>GSAAIIPPWLNIPENSRFFVIKSSSLKHVKRSF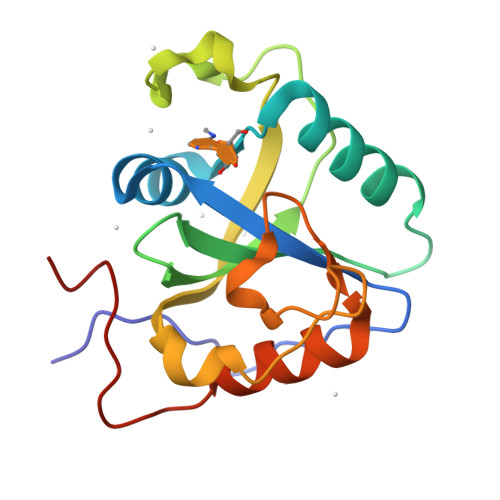YNGIWSSTHFGNKRLSEAYKKLNSGAKVFLFFSINTSGRFCGVAEMVSDLKMDLDTSIWEDEQKYGKAFKVRWVIVRDINNRSLKRFLIPSNEMKPITHSRDTQEIPYSIGISIINLFKTQDSDIFSFLDETYE[2x]In this work, we exhaustively probe the ability of all 36 immobile HJ sequences to form DNA crystals in two different designed systems. Three separate self-assembling DNA crystal systems are described in this report: the “4 × 5” and “4 × 6” designs (collectively referred to as the 4 × N systems), and a third construct with a “scrambled” sequence variant of the 4 × 6 lattices. Self-assembly was mediated by three constituent oligonucleotides: (S1) containing four sequence repeats of either 5 or 6 bases; (S2) composed of 21 bases containing complementary regions to both (S1); and (S3) which forms the second junction crossover. The HJ serves as the fundamental component at the core of each unit, and the ultimate assembly of the full lattice is facilitated by the complementary 2-base sticky ends that tail each duplex.

Seventeen of the 36 junctions successfully crystallized, a 47% success rate. Unlike the 4 × 5 motif, nearly all of the 4 × 6 junction sequences had a strong preference for crystallization in buffers containing ≥2.0 M salts (e.g., LiCl, Li2SO4, KCl, and NaCl), with the majority preferring slightly basic pH conditions in cacodylic acid. The average cell constants for the P32 crystals were a = b = 68.29 Å c = 55.68 Å. The c-axis, in particular, was ~5 Å shorter, and had a much larger degree of variability (σ = 1.97), than those that crystallized using the 4 × 5 motif. The broad range of the short axis spanned from 52.77 to 60.36 Å, and we posit that the flexible axis lengths could be responsible for rendering a larger number of junctions fatal than the 4 × 5 system. The average junction angles of 54.60° (σ = 1.44) and 58.37° (σ = 2.3) for the P32 and R3 symmetries, respectively, along with their preference for salts or organic solvents, were likely the major contributing factors that yielded the divergent lattices. However, in the majority of the crystal structures reported here, the cacodylate anion indeed fits best into the electron density map of our X-ray structures, due to the presence of sodium cacodylate in the crystallization solution.

> GAGCAGACCAGA;> CGTCACTCA;> TCTACG;> TCTGAGTGGGTCTGC> MSSSSPGEPLEPTDQDLDVLLKNLGNLVTPMALRVAATLRLVDHLLAGADTLAGLADRTDTHPQALSRLVRHLTVVGVLEGGEKQGRPLRPTRLGMLLADGHPAQQRAWLDLNGAVSHADLAFTGLLDVVRTGRPAYAGRYGRPFWEDLSADVALADSFDALMSCDEDLAYEAPADAYDWSAVRHVLDVGGGNGGMLAAIALRAPHLRGTLVELAGPAERARRRFADAGLADRVTVAEGDFFKPLPVTADVVLLSFVLLNWSDEDALTILRGCVRALEPGGRLLVLDRADVEGDGADRFFSTLLDLRMLTFMGG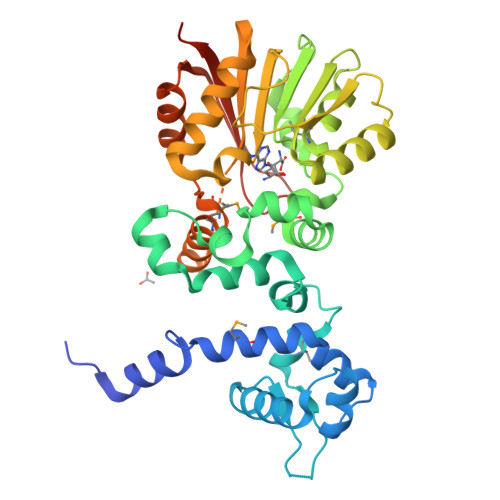RVRTRDEVVDLAGSAGLALASERTSGSTTLPFDFSILEFTAVSEEAAPAAQASEALPAQE> MKGKMAIVISTLNNPWFVVLAETAKQRAEQLGYEATIFDSQNDTAKESAHFDAIIAAGYDAIIFNPTDADGSIANVKRAKEAGIPVFCVDRGINARGLAVAQIYSDNYYGGVLMGEYFVKFLKEKYPDAKEIPYAELLGILSAQPTWDRSNGFHSVVDQYPEFKMVAQQSAEFDRDTAYKVTEQILQAHP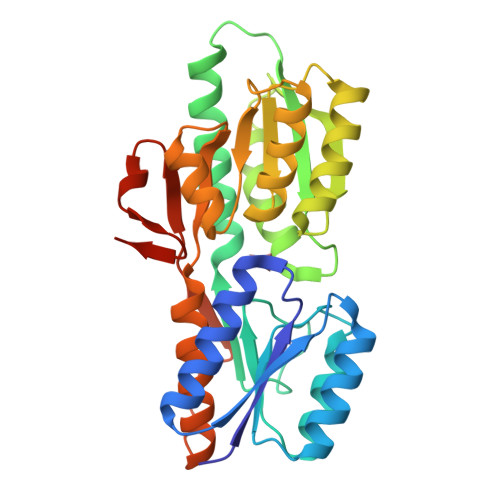EIKAIWCGNDAMALGAMKACEAAGRTDIYIFGFDGAEDVINAIKEGKQIVATIMQFPKLMARLAVEWADQYLRGERSFPEIVPVTVELVTRENIDKYTAYGRKEEGSHHHHHH>MQFPQLDPATLAAFSAAFRGELIWPSDADYDEARRIWNGTIDRRPALIARCTSTPDVVAAVSFARKSGLLVAVRGGGHSMAGHSVCDGGIVIDLSLMNSIKVSRRLRRARAQGGCLLGAFDTATQAHMLATPAGMVSHTGLGGLVLGGGFGWLSRKYGLSIDNLTSVEIVTADGGVLTASDTENPDLFWAVRGGGGNFGVVTAFEFDLHRVGPVRFASTYYSLDEGPQVIRAWRDHMATAPDELTWALYLRLAPPLPELPADMHGKPVICAMSCWIGDPHEGERQLESILHAGKPHGLTKATLPYRALQAYSFPGA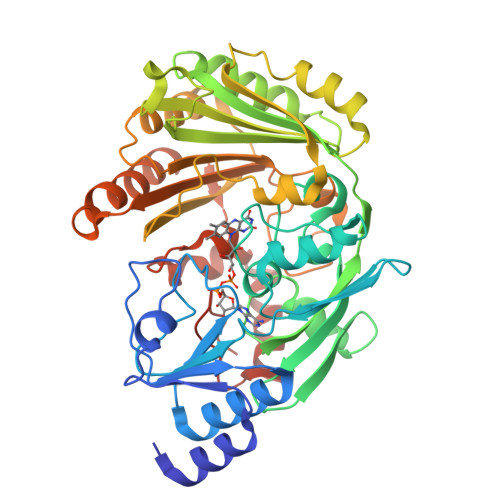VVPDRIYTKSGYLNELSDEATDTVLEHAADIASPFTQLELLYLGGAVARVPDDATAYPNRQSPFVTNLAAAWMDPTEDARHTAWAREGYRALAGHLSGGYVNFMNPGEADRTREAYGAAKFERLQGVKAKYDPTNLFRLNQNIPPSSP[4x]>MAVLSSADRASNEKKVKSSYFDLPPMEMSVAFPQATPASTFPPCTSDYYHFNDLLTPEEQAIRKKVRECMEKEVAPIMTEYWEKAEFPFHITPKLGAMGVAGGSIKGYGCPGLSITANAIATAEIARVDASCSTFILVHSSLGMLTIALCGSEAQKEKYLPSLAQLNTVACWALTEPDNGSDASGLGTTATKVEGGWKINGQKRWIGNSTFADLLIIFARNTTTNQINGFIVKKDAPGLKATKIPNKIGLRMVQNGDILLQNVFVPDEDRLP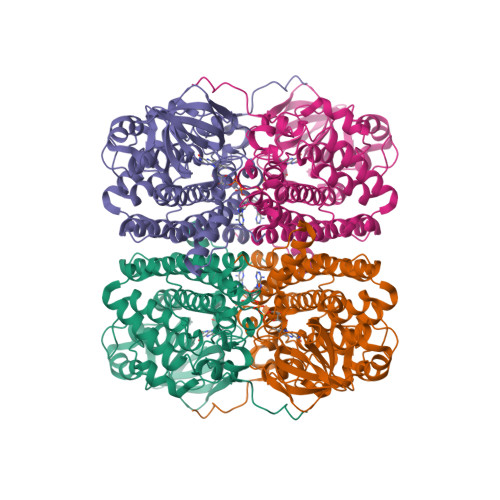GVNSFQDTSKVLAVSRVMVAWQPIGISMGIYDMCHRYLKERKQFGAPLAAFQLNQQKLVQMLGNVQAMFLMGWRLCKLYETGQMTPGQASLGKAWISSKARETASLGRELLGGNGILADFLVAKAFCDLEPIYTYEGTYDINTLVTGREVTGIASFKPATRSRLDDDGKLEHHHHHH[6x]>SNAQFRHLPMPFHWKQEELKFKTGLRRLQHRVGEIHLLREALQKGAEAGQVSLHSLIETPANGTGPSEALAMLLQETTGELEAAKALVLKRIQIWKRQQQLAGNGAPFEESLAPLQERCESLVDIYSQLQQEVGAAGGELEPKTRASLTGRLDEVLRTLVTSCFLVEKQPPQVLKTQTKFQAGVRFLLGLRFLGAPAKPPLVRADMVTEKQARELSVPQGPGAGAESTGEIINNTVPLENSIPGNCCSALFKNLLLKKIKRCERKGTESVTEEKCAVLFSASFTLGPGKLP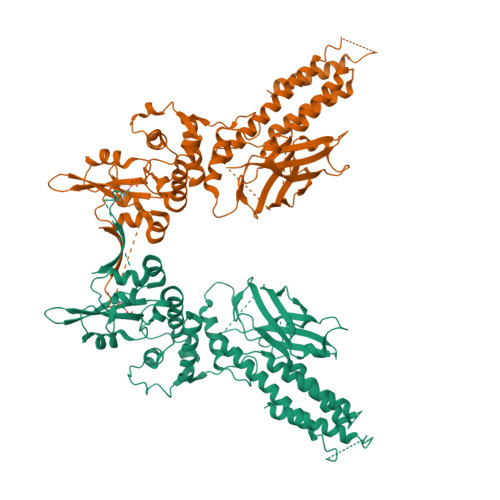IQLQALSLPLVVIVHGNQDNNAKATILWDNAFSEMDRVPFVVAERVPWEKMCETLNLKFMAEVGTNRGLLPEHFLFLAQKIFNDNSLSMEAFQHRSVSWSQFNKEILLGRGFTFWQWFDGVLDLTKRCLRSYWSDRLIIGFISKQYVTSLLLNEPDGTFLLRFSDSEIGGITIAHVIRGQDGSPQIENIQPFSAKDLSIRSLGDRIRDLAQLKNLYPKKPKDEAFRSHYKPEQMGKDGRGYVPATIKMTVERDQPLPT[2x]> SPFSVKVGLAQMLRGGVIMDVVNAEQARIAEEAGACAVMALE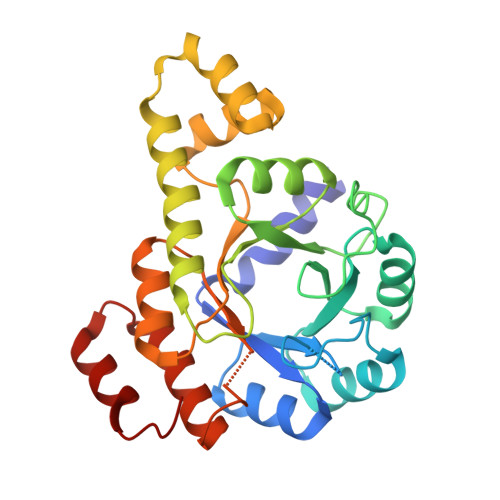RVPADIRAQGGVARMSDPQMIKEIKQAVTIPVMAKARIGHFVEAQILEAIGIDYIDESEVLTLADEDHHINKHNFRIPFVCGCRNLGEALRRIREGAAMIRTKGEAGTGNIIEAVRHVRSVNGDIRVLRNMDDDEVFTFAKKLAAPYDLVMQTKQLGRLPVVQFAAGGVATPADAALMMQLGCDGVFVGSGIFKSGDPARRARAIVQAVTHYSDPEMLVEVSCGLGEA>MRNKIFISHATPEDDDFTRWLSLKLIGLGYEVWCDILFLDKGVDFWSTIEKEIRENTCKFLIVSSTAGNKREGVLKELAVATKVKKHLQDDMFIIPLAIDENLSYDDINIEIVRLNAIDFKKSWAKGLQDLLDAFEKQNVPKKPPDHSKSNLLYQQIFLHDKQAIEKEETYDSNWFPIISFPNELRFHRYDWRLPKQFDVRTLAFPAIRYKEYLCTFAWEYDFIHQLPKTETYNGQESIRISTSDILSGRYDTDFIRNYECQRLIVQLINKAFELRMKDKNVREYQMSKTFAYWIEKGKLEKDKFEKIKLVGKQKNKYWHFGISAAGKLYPSPVLMVSSHIIFTMDGINLIKSKSIQHSSRRKQGKNWWNDKWREKLLAFIRFLSDDQNAIYLNVGSEEKILISNKPLKFFGKMSYVTPSEVTLEEESVLADINNFEEDTEDLDELEDIE[4x];>MKELIYIEEPSILFAHGQKCTDPRDGLALFGPLNQIYGIKSGVVGTQKGLQIFKSYLDKIQKPIYNHNNITRPMFPGFEAVFGCKWESQNIVFKEITDEEIRRYLFNASTHKRTYDLVTLFNDKIITANKNDEERVDVWFVIVPEEIYKYCRPNSVLPNELVQTKSLISKSKAKSFRYTPTLFEEFNKKLKEVEKEAKTYNYDAQFHDQLKARLLEHTIPTQILRESTLAWRDFKNTFGAPIRDFSKIEGHLAWTISTAAYYKAGGKPWKLGDIRPGVCYLGLVYKKIEKSKNPQNACCAAQMFLDNGDGTVFKGEVGPWYNPEKGEYHLKPKEAKALLTQALESYKEQNKSYPKEVFIHARTRFNDEEWNAFNEVTPKNTNLVGVTITKSKPLKLYKTEGAFPIMRGNAYIVDEKKAFLWTLGFVPKLQSTLSMEVPNPIFIEINKGEAEIQQVLKDILALTKLNYNACIYADGEPVTLRFANKIGEILTASTEIKTPPLAFKYYI[4x]

One new defense system is the short prokaryotic Argonaute TIR-APAZ (SPARTA), which is activated by foreign (plasmid) DNA to unleash its TIR domain for NAD(P)+ hydrolysis. The resulting depletion of the essential metabolite NAD(P)+ lends to the killing of the infected cell (abortive infection) as a means to prevent the spread of the invading DNA to the remaining bacterial cell population. The SPARTA system was first discovered in 20186 and further characterized by Koopal et al3 in 2022, who showed in an elegant set of studies that the short p-Ago of SPARTA associates with a TIR-APAZ protein to form a catalytically inactive heterodimer with 1:1 stoichiometry. However, upon guide (g) RNA and target (t) ssDNA binding, four heterodimers transition to an oligomer (a tetramer of heterodimers) that unleashes the NAD(P)ase activity of the TIR domain for abortive infection.

The cryo-EM structure of SPARTA in the presence of the gRNA/tDNA reveals four SPARTA heterodimers (A, B, C and D) assembled into a tetramer of heterodimers. The oligomer resembles a butterfly, with the MID, PIWI and APAZ domains on the outside (“wings’) and the TIR domains on the inside (the “body”). Each SPARTA heterodimer binds a single gRNA/tDNA duplex via their MID, PIWI and APAZ domains. The gRNA/tDNA duplex as a whole is accommodated in a channel that runs between the MID-PIWI and the APAZ domains. In addition, a Mg2+ ion is observed in the MID binding pocket that is coordinated to the 5’ phosphate, A3 phosphate, and Asn468 (and putatively to the main chain carbonyl of Ile507). Another major conformational change is the C-terminal terminal helix (αN) of APAZ-L2, which is ousted from its Apo position to allow binding of the 3’-end of the target DNA strand. Loop8-9 both lengthens and extends (towards α10) and residues Asp306 and Asp309 move >10 Å from their position in the Apo structure to demask the positively charged pocket for dimerization. Thus, whereas the TIR domains of heterodimers A and C are in the same orientation as in the Apo heterodimer, the TIR domains of heterodimers B and D rotate from their positions in the Apo heterodimer by ~175o in the active oligomer. Interactions between TIRA and TIRB as well as TIRC and TIRD are by mediated by a BE interface, involving residues from the BB loop of TIRB or TIRD and residues from βD, βE and αE of TIRA or TIRC. Further, TIRA-TIRB are related to TIRC-TIRD by screw-like symmetry resulting in a TIR assembly akin to the “parallel-strands” arrangement observed in scaffolding proteins (Myd88 and MAL, for example) as opposed to the “antiparallel-strands” arrangement of TIRs in enzymatic proteins (SARM1 and RPP1, for example)21.3,3'-dimethyl-1,1'-biphenyl | C14 H14 | 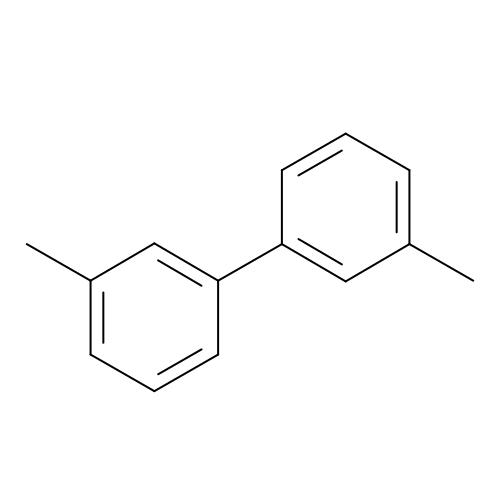GVEDOIATHPCYGS-UHFFFAOYSA-N>DSLKWIVFLLFLIVLLQL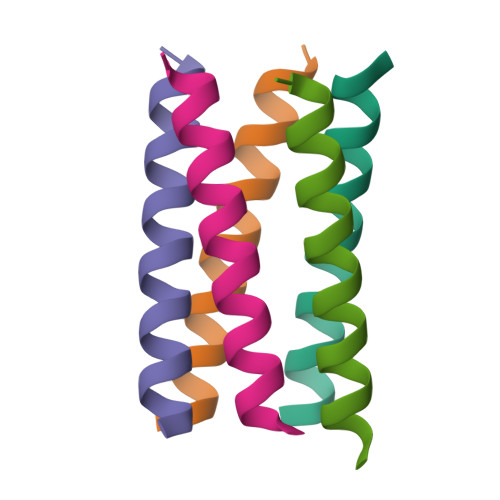AIVFLLRG[10x]> MECFVPLRCDLDGSNIEQLRQSHLSRKFIIFDEQLNLWLWFQGNSQENKRFVLQNMIILINEAQVTRTSTIDDYFTQVENNENLWRLKNDCCSKILFKSNVVMNNGYNNQIKFVFEYKSVDANFNNQDSLQDPQAKYTLDKYSSEEILPSFEPVYSWSSAATKSSKNTNNHLEKNNRATHRVSSKNSEVHEADVSRNPNTFTLKLQYPIFSLLNMRLRNISLKSEHCILSSLDFQTSKASEQLTKKFIYPQEHNSFLKLNFQEISYKLIDGTSQIELDPICPLKVPLTAFSYDS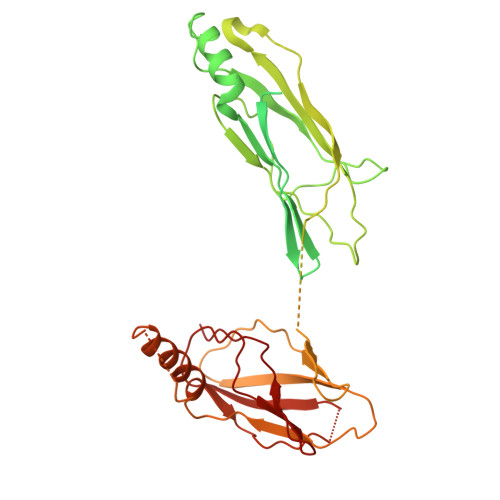ISATFKLVLLPKSTQPHRVKITLAYELELHPNLKLPVRTSWETEVTLKRSMPISSTSSQYSSNNNNTNHSASFNGAANNVNSGGLANLRLGGVSSSRFSLGAASTTSLVNSKLSNVKFKFINSNIKVIKGEKFTMRLQIINSSSSPLDLVVYYNNTINPIPSANNVRNSNGINNCGMNNGTIPNSPLTLENQYQLHNKYRKIAEGIILLSNDYKIPVVPPRETYFADLRFIGIMSGYYGTLSGLKVLDLNTNELIEVGNGASVLIQ>GALPDLKIEKLEEGVFVHTSFEEVNGWGVVTKHGLVVLVNTDAYLIDTPFTATDTEKLVNWFVERGYEIKGTISSHFHSDSTGGIEWLNSQSIPTYASELTNELLKKSGKVQAKYSFSEVSYWLVKNKIEVFYPGPGHTQDNLVVWLPESKILFGGCFIKPHGLGNLGDANLEAWPKSAKILMSKYGKAKLVVSSHSEKGDASLMKRTWEQALKGLKESKKTSSPSN[2x]

IMP-13, a member of subgroup 2, sharing 92.3% amino acid sequence similarity with IMP-2 and 82.5% with IMP-1 (Fig. SI2), was first identified in the Gram-negative pathogen Pseudomonas aeruginosa from clinical samples in Italy and is a common cause of carbapenem resistance, often involved in large outbreaks. Imipenemases represent one of the major groups of class B1 metallo-β-lactamases found in Gram-negative pathogens, and these enzymes can hydrolyze all bicyclic β-lactam antibiotics. The overall protein architecture of the IMP-13 apo structure is consistent with that of the previously published metallo-β-lactamase fold, consisting of a global αβ/βα topology with a shallow active-site cleft at the border of the two β-sheets. The structural information and dynamics presented here reveal important information about the mechanism of antibiotic binding, as well as a significant role for the active-site-covering loop (L1), indicating that the plasticity of the active-site region is important for the broad substrate recognition spectrum of these enzymes.

In complex with each of the hydrolyzed carbapenems, this loop forms a tightly locked, tunnel-like structure around the hydrolyzed antibiotic, with several hydrophobic interactions appearing to stabilize this state. The pyrrolidine ring of meropenem, doripenem, and ertapenem is suitably located to form aromatic, π-alkyl interactions with His197 and is further stabilized by the hydrophobic environment created by Val25 and Val31. In the X-ray structures, the interaction of bound ertapenem and meropenem with the Trp28 side chain occurs via the sulfur adjacent to the β-lactam ring and, additionally, via the methyl group on the pyrroline ring. Compared to the apo structures, the zinc ions in carbapenem-bound IMP-13 are located slightly farther apart, with the distance for the different antibiotics ranging from 3.8 Å (doripenem complex) to 4.2 Å (ertapenem complex), whereas the distance is 3.5 Å for the apo state, presumably to maximize interactions with the ligand. To further understand the role of the L1 loop in antibiotic binding, NMR spectra were acquired for IMP-13 in the apo state and for IMP-13 bound to ertapenem. However, notably lower values were recorded in the L1 loop in the apo state, with values of 0.51 and 0.46 for residues Asn26 and Gly29, respectively, whereas in the ertapenem-bound state, the values did not drop below 0.6 in this region. Most significantly, Trp28 NεHε had a hetNOE of 0.3 in the apo form, which rose to 0.77 in the ertapenem-bound state, comparable to the values for the backbone amides in structured regions of the protein, indicating a significant change in dynamic properties. This suggests that in the apo form the L1 loop is undergoing fast-timescale motions, while binding of antibiotic in the active site stabilizes the L1 loop.>MAHMSVIQDDYVKQAEQVIRGLPKKNGDFELTTTQLRVLLSLTAQLFDEAQLSSDQNLSPALRDKVQYLRVRFVYQAGREKAVRVFVERAGLLDELAQIGDSRDRLLKFCHYMEALVAYKKFLDPKETSKETE[5x];>[6x]MAHMTTSYAKIEITGTLTVLTGLQIGAGDGFSAIGAVDKPVVRDPLSRLPMIPGTSLKGKVRTLLSRQYGADTETFYRKPNEDHAHIRRLFGDTEEYMTGRLVFRDTKLTNKDDLEARGAKTLTEVKFENAINRVTAKANLRQMERVIPGSEFAFSLVYEVSFGTPGEEQKASLPSSDEIIE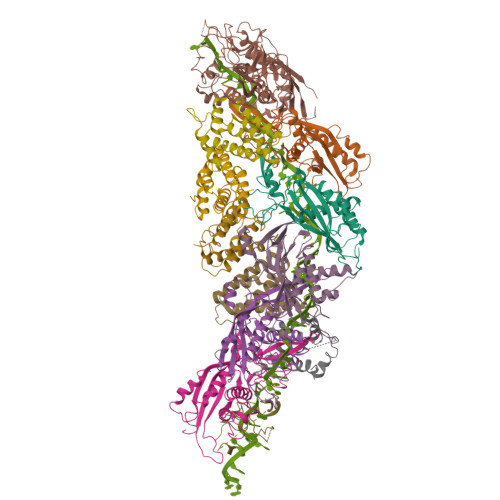DFNAIARGLKLLELDYLGGSGTRGYGQVKFSNLKARAAVGALDGSLLEKLNHELAAV;> MAHMNTYLKPFELTLRCLGPVFIGSGEKRTSKEYHVEGDRVYFPDMELLYADIPAHKRKSFEAFVMNTDGAQATAPLKEWVEPNAVKLDPAKHRGYEVKIGSIEPRRASRGRGGRMTRKKLTLNEIHAFIKDPLGRPYVPGSTVKGMLRSIYLQSLVHKRTAQPVRVPGHQTREHRQYGERFERKELRKSGRPNTRPQDAVNDLFQAIRVTDSPALRTSDLLICQKMDMNVHGKPDGLPLFRECLAPGTSISHRVVVDTSPTARGGWREGERFLETLAETAASVNQARYAEYRAMYPGVNAIVGPIVYLGGGAGYRSKTFVTDQDDMAKVLDAQFGKVVKHVDKTRELRVSPLVLKRTKIDNICYEMGQCELSIRRAE> GDPIADMIDQTVNNQVNRSLTALQVLPTAANTEASSHRLGTGVVPALQAAETGASSNASDKNLIETRCVLNHHSTQETAIGNFFSRAGLVSIITMPTTGTQNTDGYVNWDIDLMGYAQLRRKCELFTYMRFDAEFTFVVAKPNGELVPQLLQYMYVPPGAPKPTSRDSFAWQTATNPSVFVKMTDPPAQVSVPFMSPASAYQWFYDGYPTFGEHLQANDLDYGQCPNNMMGTFSIRTVGTEKSPHSITLRVYMRIKHVRAWIPRPLRNQPYLFKTNPNYKGNDIKCTSTSRDKITTL;> SPSAEACGYSDRVAQLTIGNSTITTQEAANIVIAYGEWPEYCPDTDATAVDKPTRPDVSVNRFFTLDTKSWAKDSKGWYWKFPDVLTEVGVFGQNAQFHYLYRSGFCVHVQCNASKFHQGALLVAVLPEYVLGTIAGGTGNENSHPPYATTQPGQVGAVLTHPYVLDAGIPLSQLTVCPHQWINLRTNNCATIIVPYMNTVPFDSALNHCNFGLLVIPVVPLDFNAGATSEIPITVTIAPMCAEFAGLRQAVKQ;> GIPTELKPGTNQFLTTDDGVSAPILPGFHPTPPIHIPGEVHNLLEICRVETILEVNNLKTNETTPMQRLCFPVSVQSKTGELCAAFRADPGRDGPWQSTILGQLCRYYTQWSGSLEVTFMFAGSFMATGKMLIAYTPPGGNVPADRITAMLGTHVIWDFGLQSSVTLVVPWISNTHYRAHARAGYFDYYTTGIITIWYQTNYVVPIGAPTTAYIVALAAAQDNFTMKLCKDTEDIEQTANIQ;> MGSQVSTQRSGSHENSNSASEGSTINYTTINYYKDAYAASAGRQDMSQDPKKFTDPVMDVIHEMAPPLK

Coxsackievirus A16 (CVA16) and enterovirus 71 (EV71) are the major causative agents of HFMD. The viral genome is enclosed in a non-enveloped icosahedral capsid that is built out of 60 copies of the structural proteins VP1 to VP4. VP1 surrounds the 5-fold axes and VP2 and VP3 alternate around the 2- and 3-fold axes, while VP4 forms part of the inner lining of the capsid. Structural analysis has revealed that each of the 60 VP1 proteins in the enterovirus capsid contain a hydrophobic ‘pocket factor’.

The crystal structure of CVA16 in complex with the uncoating inhibitor GPP3 was determined by crystallography. To this end, CVA16 crystals were soaked with the inhibitor dissolved in DMSO because GPP3, like most pocket-factor analogs, is rather insoluble in water. Data were scaled together, merged and the structure solved at 2.75 Å resolution by molecular replacement using the structure of the mature CVA16 virus. The electron density map revealed that the compound replaces the natural pocket factor (modeled as sphingosine) with only a negligible shift (~ 0.2 Å) in the polypeptide backbone of the residues lining the pocket, reflecting its shape similarity with sphingosine. The surface area accessible to solvent, calculated by Areaimol, is 12.3 Å2 for GPP3 in the VP1 pocket whereas for the sphingosine it is 11.8 Å2. This demonstrates that GPP3 is buried within the pocket. As expected, GPP3 binds with its pyridine ring close to the entrance of the pocket, with the carbonyl oxygen of the imidazole moiety hydrogen-bonding to the backbone nitrogen of residue Ile113, which is also the case for sphingosine, and with the phenoxy ring sandwiched between two hydrophobic residues (Phe135 and Tyr155). This binding mode was also observed for EV71 in complex with the same compound, except that EV71 has a phenylalanine at position 155. The docking of GPP3 in the crystal structure reproduces exactly the experimentally observed pose with an energy of interaction of -66 Kcal/mol, expressed as a sum of van der Waals and electrostatic energies. We investigated the interaction of GPP3 with CVA16 by determining the crystal structure of it in complex with the whole virus particle and identified the key residues involved in the interactions with the capsid binder including Phe135 and Tyr155 which make a hydrophobic sandwich with the phenoxy moiety as observed for EV71.>GGGACAAGUUCCCGAAAGGAUGGCGGAAACGCCAGAU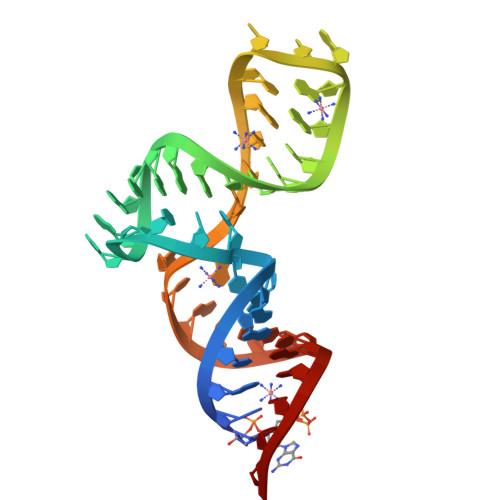GCCUUGUCCC[2x]>AAAGGGGAGUAGCGUCGGGAAACCGAAACAAAGUCGUCAAUUCGUGAGGAAACUCACCGGCUUUGUUG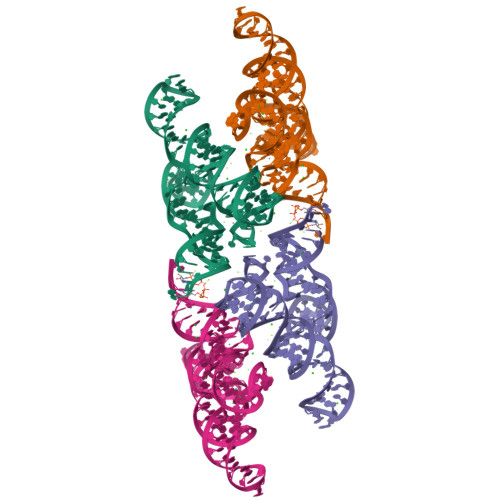ACAUACGAAAGUAUGUUUAGCAAGACCUUUCC[2x]Cephalosporins are members of the β-lactam family of antibiotics. These drugs achieve their bactericidal potency by irreversibly inhibiting penicillin-binding proteins (PBPs), particularly the transpeptidase (TPase) PBPs that cross-link cell wall peptidoglycan. Four annotated TPase PBPs exist in the genome of C. difficile R20291, a hypervirulent epidemic ribotype 027 strain: PBP1 (CDR20291_0712), PBP2 (CDR20291_0985), PBP3 (CDR20291_1067), and SpoVD (CDR20291_2544). A recent study found PBP1 and PBP2 are essential for vegetative growth in R20291, while SpoVD and PBP3 are essential for sporogenesis. Remarkably, in addition to C. difficile PBP2, we find this Zn2+-binding motif is also present in C. difficile PBP3 and SpoVD, meaning three of the four TPase PBPs, and all three class B PBPs in C. difficile have this motif.

Next, we determined the structures of PBP3 and SpoVD, at 2.40 Å and 2.20 Å resolution. Both SpoVD and PBP3 possess a canonical class B PBP fold that closely resembles Pseudomonas aeruginosa and E. coli PBP329,30. Like PBP2, the four residues in the Zn2+-binding motif of C. difficile PBP3 and SpoVD consist of an invariant His, a Cys from the X residue of the SXN motif, and two electron rich residues—in this case Cys instead of Asp. Importantly, we find Zn2+ binds in an almost identical manner as PBP2, suggesting Asp and Cys are interchangeable at the first and second position. The significance of the Asp → Cys substitution between SpoVD/PBP3 and PBP2 is unclear. Whereas the redox-sensitive cysteine in the SXN motif for PBP2 can potentially function as a sensor for environmental oxygen levels, the replacement of Asp for Cys in both sporulation specific PBPs (PBP3 and SpoVD) may further enhance the sensitivity and/or subject them to additional regulation. Subsequent biochemical analysis of purified PBP1, PBP2, and PBP3 demonstrate PBP1 and PBP2 are selectively insensitive to most cephalosporins, in contrast to the non-essential PBP3 which is potently inhibited by all β-lactams. Nonetheless, SpoVD and PBP3 are very promising drug targets.

> GDKYKQSVESQSVEKVELNSGRGIIYDRNNKKLTDTSKSQVLIVEKEKLNNNYKILELIKKATKMNDLDIYKAVQEQLTRPIIQIQTKNIDKSMKKELEKNGIMVEEKTMRYAKDGLLSHTIGYIKEDDKSGQSGIEKSMDSVLRNSNEKYISAFKAGDAGNEKSLNILKGSVKTVDNKDKDRHLKTTIDYNIQKKLEQILNKEENPTAAIISEASTGEILAMCSRPNFDQNDISKSLKGKNGEFENRVIKATYPPGSVFKMVVLFSALENGVIDENYTYNCTGKTKVGNTNEILRCNKRDGHGFQNLRQAFSNSCNPAFLDIAMKLGKEKILKSAEKLHLFEKVDIGLDEEKIREAPKNISIRNLAIGQENIEFTPLQINQMTQIIANNGTFKPLYLYKSLVDNNMNTIKTYKSSKKEELISPYVCTQVKEYMKSVSRIGTAKDLKDIEGGCGVKTGTAQSSLNKKAIDHGWITGFYPEERPKYVITVLVEGTQKGNKSATPIFKEICESIK Human dipeptidyl peptidase III (hDPP III), also known as enkephalinase B, is a member of the M49 family of zinc dependent metallopeptidases and cleaves dipeptides sequentially from the N-terminus of various bioactive peptide substrates. Crystal structures have so far been determined for DPP III from humans as well as from Saccharomyces cerevisiae. Despite the low sequence identity (36%) shared by the two proteins, both structures are very similar and consist of two lobes separated by a wide cleft. The “upper” lobe is mostly α-helical and contains the zinc binding site as well as the catalytically important residues. In both structures, two histidine residues (His-450 and His-455 in the human enzyme) and a glutamate (Glu-508) coordinate the zinc ion.

Met-enkephalin (YGGFM) and Leu-enkephalin (YGGFL) are endogenous opioid neurotransmitters which are found in the brains and spinal cords of many animals, including humans, and which have been shown to be cleaved by hDPP III1. In addition, Leu-enkephalin has been shown to bind to the inactive hDPP3 variant with a Kd of 3.6 μM17. In the complex structures, the N-termini of both peptides are anchored to the protein through hydrogen bonding and electrostatic interactions from the side chains of Tyr-318, Glu-316 and Asn-394. The first three amino acids form a β-strand, which interacts with the five-stranded β-core in an antiparallel fashion (through hydrogen bonds to Ala-388 to Asn-391). One exception is His-568 from the upper lobe, which is hydrogen bonded to the carbonyl oxygen of the scissile peptide bond. In the complex with Leu-enkephalin an additional residue (Arg-572) from the upper lobe forms a hydrogen bond with of Phe-4 of the peptide (3.3 Å). In both complexes the C-terminal residue (Met or Leu) appears to be quite flexible as indicated by weaker electron density in this region. Quite unexpectedly, the zinc ion does not directly interact with the P1 carbonyl of the peptide (the scissile peptide) but is at a distance of 3.7 Å and 3.6 Å for Met and Leu-enkephalin, respectively. Instead, a water molecule completes the tetrahedral coordination of the metal ion. When analysing the interactions with the catalytic zinc ion, we observed that the carbonyl group of the scissile peptide bond is not directly interacting with the catalytic zinc ion (3.7 Å distance) in the complexes with Met- and Leu-enkephalin and a water molecule is bound to the ion.

> MADTQYILPNDIGVSSLDSREAFRLLSPTERLYAYHLSRAAWYGGLAVLLQTSPEAPYIYALLSRLFRAQDPDQLRQHALAEGLTEEEYQAFLVYAAGVYSNMGNYKSFGDTKFVPNLPKEKLERVILGSEAAQQHPEEVRGLWQTCGELMFSLEPRLRHLGLGKEGITTYFSGNCTMEDAKLAQDFLDSQNLSAYNTRLFKEVDGCGKPYYEVRLASVLGSEPSLDSEVTSKLKSYEFRGSPFQVTRGDYAPILQKVVEQLEKAKAYAANSHQGQMLAQYIESFTQGSIEAHKRGSRFWIQDKGPIVESYIGFIESYRDPFGSRGEFEGFVAVVNKAMSAKFERLVASAEQLLKELPWPPTFEKDKFLTPDFTSLDVLTFAGSGIPAGINIPNYDDLRQTEGFKNVSLGNVLAVAYATQREKLTFLEEDDKDLYILWKGPSFDVQVGLHALLGHGSGKLFVQDEKGAFNFDQETVINPETGEQIQSWYRCGETWDSKFSTIASSYEECRAESVGLYLSLHPQVLEIFGFEGADAEDVIYVNWLNMVRAGLLALEFYTPEAFNWRQAHMQARFVILRVLLEAGEGLVTITPTTGSDGRPDARVRLDRSKIRSVGKPALERFLRRLQVLKSTGDVAGGRALYEGYATVTDAPPESFLTLRDTVLLRKESRKLIVQPNTRLEGSDVQLLEYEASAAGLIRSFSERFPEDGPELEEILTQLATADARFW;> YGGFL> AMCIPLWPARNGNTAHLVMCPFAGGSSSAFRHWQAEQLADCALSLVTWPGRDRLRHLEPLRSITQLAALLANELEASVSPDTPLLLAGHAMGAQVAFETCRLLEQRGLAPQGLIISGCHAPHLHSERQLSHRDDADFIAELIDIGGCSPELRENQELMSLFLPLLRADFYATESYHYDSPDVCPPLRTPALLLCGSHDREASWQQVDAWRQWLSHVTGPVVIDGDHFYPIQQARSFFTQIVRHFPHA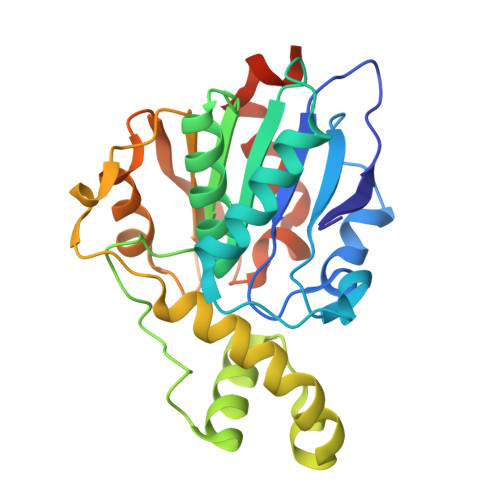FSAMTAWQKQPSTSER> MLSRKGIIPEEYVLTRLAEDPTEPRYRTRERRARFVSKKGNCNVAHKNIREQGRFLQDVFTTLVDLKWPHTLLIFTMSFLCSWLLFAMVWWLIAFAHGDLAPGEGTNVPCVTSIHSFSSAFLFSIEVQVTIGFGGR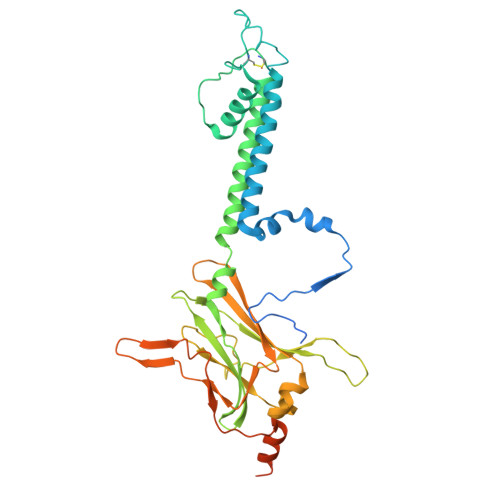MVTEECPLAILILIVQNIVGLMINAIMLGCIFMKTAQAHRRAETLIFSKHAVITPRHGRLCFMLRVGDLRKSMIISATIHMQVVRKTTSPEGEVVPLHQVDIPMENGVGGNSIFLVAPLIIYHVIDSNSPLYDLAPSDLHHHQDLEIIVILEGVVETTGITTQARTSYLADEILWGQRFVPIVAEEDGRYSVDYSKFGNTVKVPTPLCTARQLDEDRSLLDALTLASSRGPLRKRSVAVAKAKPKFSISPDSLS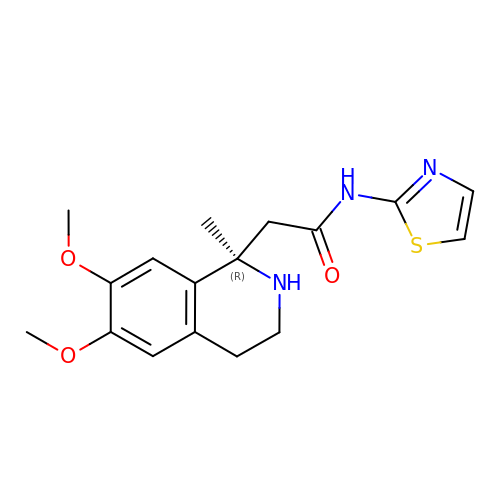2-[(1R)-6,7-dimethoxy-1-methyl-1,2,3,4-tetrahydroisoquinolin-1-yl]-N-(1,3-thiazol-2-yl)acetamide | C17 H21 N3 O3 S | GGTAOAOMAPVDLB-QGZVFWFLSA-N> MNARSTGQHPARYPGAAAGEPTLDSWQEPPHNRWAFAHLGEMVPSAAVSRRPVNAPGHALARLGAIAAQLPDLE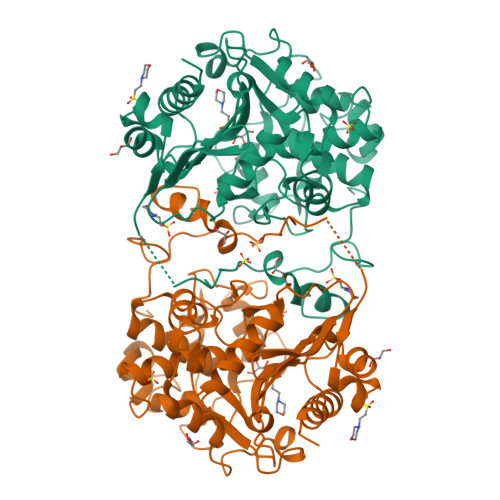QRLEQTYTDAFLVLRGTEVVAEYYRAGFAPDDRHLLMSVSKSLCGTVVGALVDEGRIDPAQPVTEYVPELAGSVYDGPSVLQVLDMQISIDYNEDYVDPASEVQTHDRSAGWSTRRHGDPADTYEFLTTLRGDGSTGEFQYCSANTDVLAWIVERVTGLRYVEALSTYLWAKLDADRDATITVDTTGFGFANGGVSCTARDLARVGRMMLDGGVAPGGRVVSEDWVRRVLAGGSHEAMTDKGFTNTFPDGSYTRQWWCTGNERGNVSGIGIHGQNLWLDPLTDSVIVKLSSWPDPYTEHWHRLQNGILLDVSRALDAV> SRPIVISGPSGTGKSTLLKKLFAEYPDSFGFSVSSTTRTPRAGEVNGKDYNFVSVDEFKSMIKNNEFI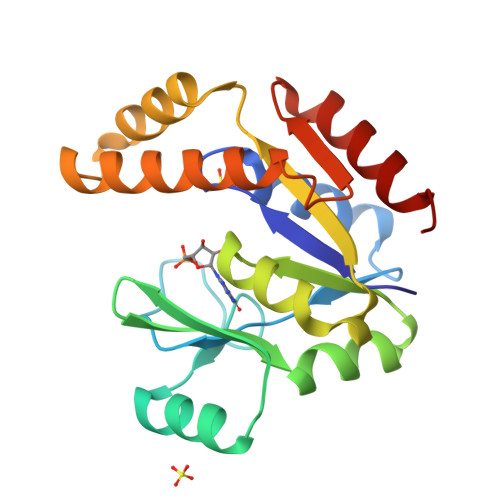EWAQFSGNYYGSTVASVKQVSKSGKTCILDIDMQGVKSVKAIPELNARFLFIAPPSVEDLKKRLEGRGTETEESINKRLSAAQAELAYAETGAHDKVIVNDDLDKAYKELKDFIFAEK>[3x]MSHPDLNKLLELWPHIQEYQDLALKHGINDIFQDNGGKLLQVLLITGLTVLPGREGNDAVDNAGQEYELKSINIDLTKGFSTHHHMNPVIIAKFRQVPWIFAIYRGIAIEAIYRLEPKDLEF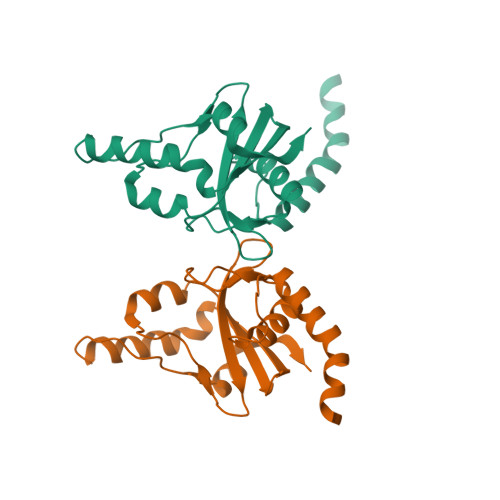YYDKWERKWYSDGHKDINNPKIPVKYVMEHGTKIYAA> ENLYFQGMKPIHVGLLGLGTVGGGTLTVLRRNAEEITRRAGREIRVVRAAVRNLDKAEALAGGLPLTTNPFDVVDDPEIDIVVELIGGLEPARELVMQAIANGKHVVTANKHLVAKYGNEIFAAAQAKGVMVTFEAAVAGGIPIIKALREGLTANRIEWLAGIINGTSNFILSEMRDKGAAFDDVLKEAQRLGYAEADPTFDIEGIDAAHKLTILSAIAFGIPMQFERAYTEGISQLTREDVRYAEELGYRIKLLGIARRAENGIELRVHPTLIPERRLIANVDGAMNAVLVKGDAVGPTLYYGAGAGSEPTASAVVADLVDVTRLHTADPHHRVPHLAFQPDQLADTPILPMEAVRTAYYLRLRAFDRPGVLADITRILA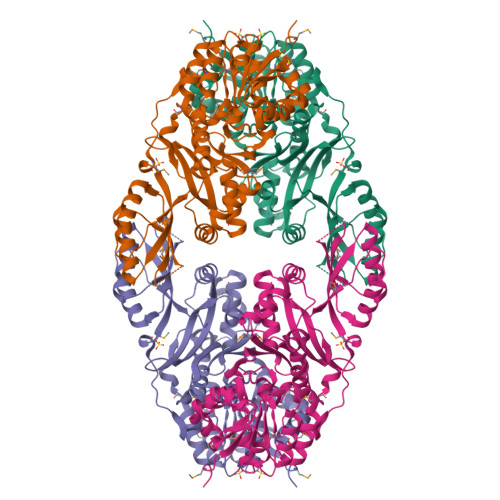DSSISIDAMVQKEPAEGEEQVDIILLTHVTLEKNVNAAIAKIEALDAVAGKVMRIRLEDLGAK>[3x]MATKGTKRSYEQMETDGERQNATEIRASVGKMIDG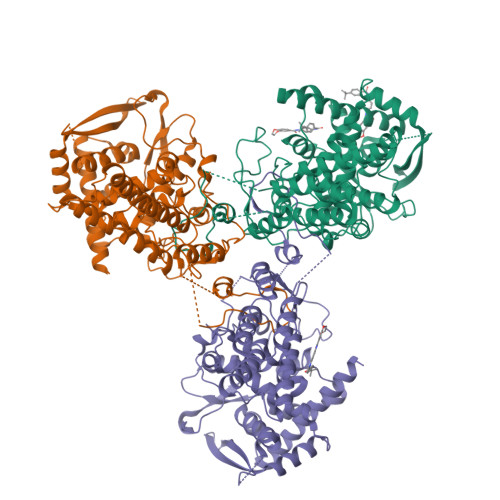IGRFYIQMCTELKLSDYEGRLIQNSLTIERMVLSAFDERRNKYLEEHPSAGKDPKKTGGPIYRRVDGKWRRELILYDKEEIRRIWRQANNGDDATAGLTHMMIWHSNLNDATYQRTRALVRTGMDPRMCSLMQGSTLPRRSGAAGAAVKGVGTMVMELIRMIKRGINDRNFWRGENGRRTRIAYERMCNILKGKFQTAAQRTMVDQVRESRNPGNAEFEDLIFLARSALILRGSVAHKSCLPACVYGSAVASGYDFEREGYSLVGIDPFRLLQNSQVYSLIRPNENPAHKSQLVWMACHSAAFEDLRVSSFIRGTKVVPRGKLSTRGVQIASNENMETMESSTLELRSRYWAIRTRSGGNTNQQRASSGQISIQPTFSVQRNLPFDRPTIMAAFTGNTEGRTSDMRTEIIRLMESARPEDVSFQGRGVFELSDEKATSPIVPSFDMSNEGSYFFGDNAEEYDN>SHMAIVKVTDADFDSKVESGVQLVDFWATACGPCKMIAPVLEELAADYEGKADILKLDVDENPSTAAKYEVMSIPTLI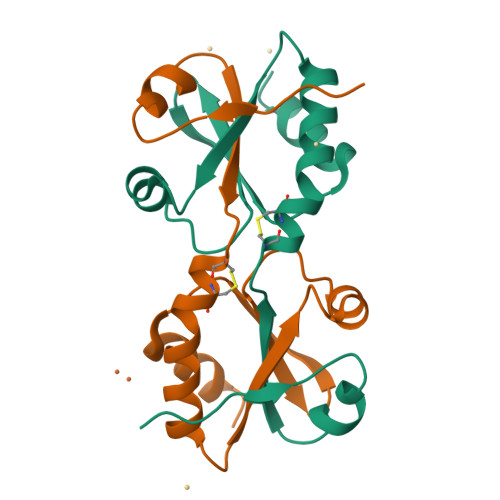VFKDGQPVDKVVGFQPKENLAEVLDKHL[2x]>MEISELEGKKVPHGEVTLVGAGRLGFRTALNLMQIHRGGPERIKVIDGQKVSADDLIFRLMGAKIGEYKVKFIESLACDGFSRTVQGIPEYITGDNLRLIGGDVVCVEIAGGDTLPITTEIIRYAQERGAATISTMGVFGIGEEDVSVVDIDEADPENPIAAYLQAEGIHEHVL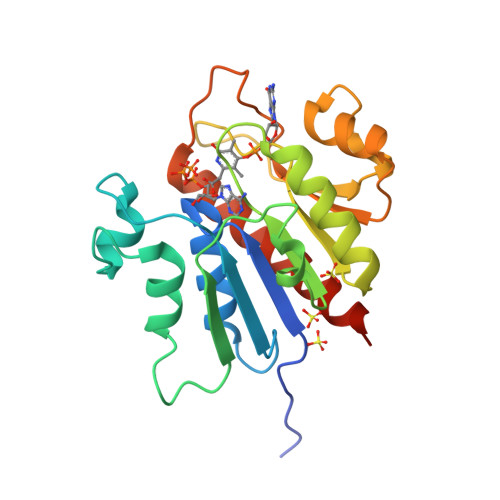VGTGKLIRDWEPVTPHVLDRVSEVMTAEILKLLRGAQRLELVPR[4x]Human Epidermal growth factor Receptor 4 (HER4 or ERBB4) carries out essential functions in the development and maintenance of the cardiovascular and nervous systems. HER4 activation is regulated by a diverse group of extracellular ligands including the neuregulin (NRG) family and betacellulin (BTC), which promote HER4 homodimerization or heterodimerization with other HER receptors. Important cardiovascular functions of HER4 are exerted via heterodimerization with its close homolog and orphan receptor, HER2. Here, we report cryo-EM structures of near full-length HER2/HER4 heterodimers and full-length HER4 homodimers bound to NRG1β and BTC.

To test this hypothesis for HER4 complexes, we determined the cryo-EM structures of full-length HER4 homodimers bound to NRG1β or BTC. In both structures, HER4 kinase domains were bound to afatinib to enable high-resolution reconstruction in the ECD module (3.4 Å for NRG1β, and 3.7 Å for BTC). We present here the first cryo-EM reconstructions of both the homodimer and heterodimer complexes of the HER4 receptor in its full-length form, bound to two different high-affinity HER4 cognate growth factors, NRG1β and BTC. This is also the first time that a betacellulin growth factor has been resolved bound to a HER receptor. The HER4/NRG1β and HER4/BTC homodimers adopt overall similar conformations, but our reconstructions show differences in the intermonomer angles that are adopted by NRG1β- vs BTC-bound homodimers. The two receptors in the HER4/NRG1β dimer adopt an angle of 37 degrees compared to 33 degrees for HER4/BTC. Detailed 3D classification analysis revealed substantial scissor-like movements around the dimerization arm in both data sets with the concerted intermonomer movement of domains I and IV, varying from 35 to 39 degrees for HER4/NRG1β and 30–35 degrees for HER4/BTC. In the HER4/NRG1β pocket, HER4 K438, K35, E112 and D376 form salt bridges with NRG1β E215, D219, R207 and R220, respectively. In the HER4/BTC pocket, HER4 D376 also engages an equivalent BTC R103, but the other three residues are substituted with hydrophobic/polar residues in BTC (NRG1β E215=BTC G98, NRG1β D219=BTC A102, NRG1β R207=BTC T90). Thus, substitutions into small, apolar residues in BTC result in a more ‘compressed’ ligand-binding pocket in HER4/BTC homodimers than in HER4/NRG1β homodimers, which may allosterically determine different intermonomer angles via modulation of dimerization arm positioning. Eight of them are resolved in the cryo-EM maps of both HER4/NRG1β and HER4/BTC homodimers that enabled the building of core glycan trees up to 5 sugar moieties (shown for HER4 /NRG1β).

>[2x]QSVCAGTENKLSSLSDLEQQYRALRKYYENCEVVMGNLEITSIEHNRDLSFLRSVREVTGYVLVALNQFRYLPLENLRIIRGTKLYEDRYALAIFLNYRKDGNFGLQELGLKNLTEILNGGVYVDQNKFLCYADTIHWQDIVRNPWPSNLTLVSTNGSSGCGRCHKSCTGRCWGPTENHCQTLTRTVCAEQCDGRCYGPYVSDCCHRECAGGCSGPKDTDCFACMNFNDSGACVTQCPQTFVYNPTTFQLEHNFNAKYTYGAFCVKKCPHNFVVDSSSCVRACPSSKMEVEENGIKMCKPCTDICPKACDGIGTGSLMSAQTVDSSNIDKFINCTKINGNLIFLVTGIHGDPYNAIEAIDPEKLNVFRTVREITGFLNIQSWPPNMTDFSVFSNLVTIGGRVLYSGLSLLILKQQGITSLQFQSLKEISAGNIYITDNSNLCYYHTINWTTLFSTINQRIVIRDNRKAENCTAEGMVCNHLCSSDGCWGPGPDQCLSCRRFSRGRICIESCNLYDGEFREFENGSICVECDPQCEKMEDGLLTCHGPGPDNCTKCSHFKDGPNCVEKCPDGLQGANSFIFKYADPDRECHPCHPNCTQGCNGPTSHDCIY;>[2x]GHFSRCPKQYKHYCIKGRCRFVVAEQTPSCVCDEGYIGARCERVDLFY>GSKKLINDVQDVLDEQLAGLAKAHPSLTLHQDPVYVTRADAPVAGKVALLSGGGSGHEPMHCGYIGQGMLSGACPGEIFTSPTPDKIFECAMQVDGGEGVLLIIKNYTGDILNFETATELLHDSGVKVTTVVID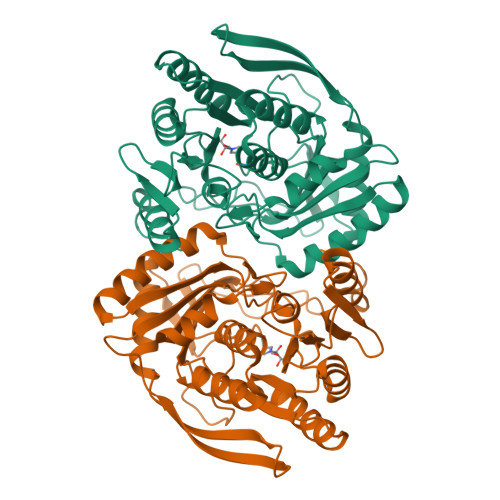DDVAVKDSLYTAGRRGVANTVLIEKLVGAAAERGDSLDACAELGRKLNNQGHSIGIALGACTVPAAGKPSFTLADNEMEFGVGIHGEPGIDRRPFSSLDQTVDEMFDTLLVNGSYHRTLRFWDYQQGSWQEEQQTKQPLQSGDRVIALVNNLGATPLSELYGVYNRLTTRCQQAGLTIERNLIGAYCTSLDMTGFSITLLKVDDETLALWDAPVHTPALNWGK[2x]>MASMTGGQQMGRGSMNKPQSWEARAETYSLYGFTDMPSLHQRGTVVVTHGEGPYIVDVNGRRYLDANSGLWNMVAGFDHKGLIDAAKAQYERFPGYHAFFGRMSDQTVMLSEKLVEVSPFDSGRVFYTNSGSEANDTMVKMLWFLHAAEGKPQKRKILTRWNAYHGVTAVSASMTGKPYNSVFGLPLPGFVHLTCPHYWRYGEEGETEEQFVARLARELEETIQREGADTIAGFFAEPVMGAGGVIPPAKGYFQAILPILRKYDIPVISDEVICGFGRTGNTWGCVTYDFTPDAIISSKNLTAGFFPMGAVILGPELSKRLETAIEAIEEFPHGFTASGHPV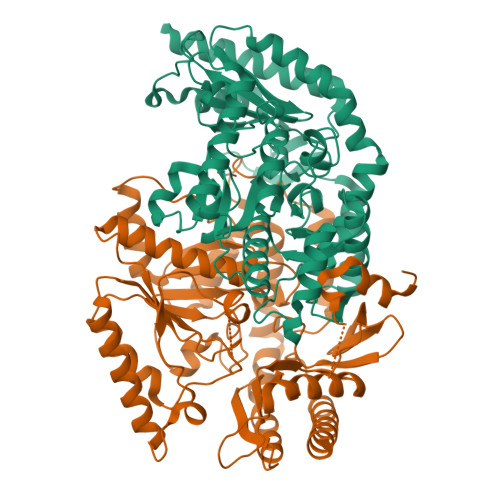GCAIALKAIDVVMNEGLAENVRRLAPRFEERLKHIAERPNIGEYRGIGFMWALEAVKDKASKTPFDGNLSVSERIANTCTDLGLICRPLGQSVVLCPPFILTEAQMDEMFDKLEKALDKVFAEVAAA[2x]>[2x]MFTTRPTLQGTFGMVSSTHWLASQSAMAVLEDGGNAYDAAVAGAFVLHVVEPHLNGPAGEVPILLAPAGGEVRVLCGQGVAPAGATVAHYKGLGLDLVPGTGPLAAAVPGAFDAWMLLLRDHGTKPLADVLKYAVGYAEHGHAPVENVGVTVETVRELFETEWTTSADVYLPGGKAPRPGELLRNPTLAATWKRLLAEVAGAGDREAQIEAAREVWRTGFIAEALVRQARRPTMDTSGERHTGTLTAADLAGWSATYEAPATYDWNGWTVCKAGPWSQGPVLLQQLALLPPELPEYGSADYVHLLVEGCKLAMADREAWYGDAAEVPLDELLSAEYNAGRRELVGDKASHELRPGSPGGRTARLSAHADLVATGEPGFDPLGAGEPTAAMGAGEPTVAKLPASPVPGEPDVAADGSTRGDTCHLDVVDRWGNMVAATPSGGWLQSNPVVPELGFPLGTRLQMTWLEEGLPNSLTPGRRPRTTLTPSIALRDGIPVMAFG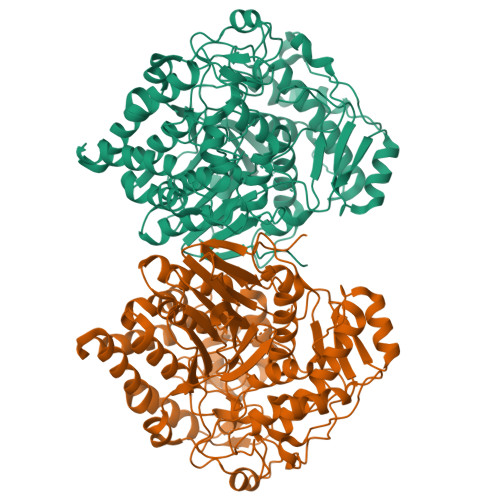TPGGDQQDQWQLHFFLAVALRARVRGGLDLQGAIDAPNWHNDSFPGSFYPRGMRPGSVTVEARMDPGIAAELRRRGHEVTVGPPWSEGRLCAVARDPRTGILSAAANPRGMQGYAVGR>G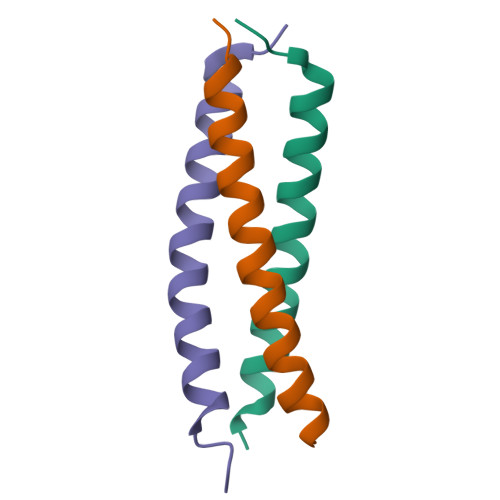GWVSGEEFYMLTRRVLQLETVLEGVVSQIDAVGSKLKM[6x]>GPTLVPTKMQVTAPANISASAQTFEVACDYNGAIATLSDDGDMVGTAIVKDGKAIIKLNESIADETNLTLTVVGYNKVTVIKDVKVEGTSIEGRAADKPYTVAVSGKTITVESPAAGLTIFDMNGRRVATAKNRMVFEAQNGVYAVRIATEGKTYTEKVIVK[2x]

The virulence of P. gingivalis is dependent on secreted cysteine proteases called gingipains (RgpA, RgpB, and Kgp) that are essential for corruption of the host immune system and acquisition of nutrients and heme – a vital growth factor and source of black pigmentation of colonies on blood agar. Gingipains are synthesized with a typical N-terminal signal peptide targeting them to the Sec translocon and are exported through the OM via a novel secretion system referred to as “Por Secretion System; PorSS” or following the naming convention, Type IX Secretion System (T9SS)7. Translocation of gingipains from the periplasm across the OM is dependent on a conserved C-terminal domain (CTD), which appears to be important for secretion of the proteins and in particular, truncation of the last few C-terminal residues of this domain leads to accumulation of gingipains in the periplasm. Here, we show for the first time that the OM translocation signal, a conserved CTD of RgpB, has a typical Ig-like fold encompassing seven antiparallel β-strands organized in two β-sheets that are packed against each other in a β-sandwich.

However, diffraction quality crystals were obtained using mutants of the same construct, which included an inserted hexahistidine after residues S664 or I665 (recombinant products r664i6H and r665i6H, respectively), or by substitution of six consecutive linker residues (I665ADVAN670) with a factor Xa cleavage motif (IEGRAA; r665sXa). The three structures were solved and refined with diffraction data to 1.9 Å, 2.4 Å, and 2.1 Å resolution, respectively. Each variant of rIgSF-CTD formed nearly identical crystal structures (RMSD of 0.760 Å for r665i6H and 0.327 Å for r665sXa, with respect to r664i6H for 298 aligned residues). In each tandem, the IgSF and CTD domains showed an orthogonal arrangement, with their longest axes tilted by 90 degrees with respect to each other. The 9-residue linker (T663-D671) between the immunoglobulin-like subdomain and the CTD did not yield visible electron density, indicating that this fragment was disordered in the crystals. The lack of cleavage observed within the linker by elastase is clearly not due to inaccessibility of this loop to proteolytic enzymes, as proteins bearing the IEGRAA motif by insertion/substitution were efficiently cleaved at the Arg-Ala peptide bond by fXa. Interestingly, however, there was a clear difference in the kinetics of cleavage events, with r662iXa being far more susceptible to proteolysis than r665sXa. Taken together, these results demonstrate that insertion and substitution within the connecting linker do not affect domain structure or inter-domain arrangement, and suggest that the linker is resistant to proteolysis despite the presence of peptide bonds potentially susceptible to cleavage by HNE and PPE.Here, we have characterized an exceptionally large microvirus, Ebor, and provide crucial insights into long-standing mechanistic questions. Here, we report the structural analysis of the genome delivery process of a Microviridae phage, Ebor, along with its discovery and characterization. This phage, infecting a model aquatic Alphaproteobacterium Rhodobacter capsulatus, belongs to the microvirus taxon ‘Tainavirinae’ and recognizes the host via five Gokushovirinae-like trimeric protrusions. The capsid exhibits the triangulation number of T=1, being made of 60 copies of the major capsid protein. The core of the major capsid protein contains an 8-stranded antiparallel β-barrel (single jelly-roll fold), the fold shared among all Microviridae.

We isolated two Ebor variants exhibiting different stability during cryo-EM sample preparation. Nanopore sequencing showed a single nucleotide polymorphism leading to S120R amino acid replacement in the major capsid protein. Thus, we designated these variants S120 and R120. Variant R120 virions were purified using CsCl gradient, vitrified and imaged using cryo-EM, yielding stable native particles. Single particle reconstruction produced an icosahedrally averaged map of Ebor at 3.2 Å resolution. The capsid shell has an external diameter of 28 nm and an internal diameter of 25.1 nm. The internal diameter is 3.2 to 4.6 nm larger compared to other determined capsid structures of Microviridae members, allowing Ebor to accommodate larger genome. A striking characteristic of the capsid is the presence of elongated protrusions situated at its three-fold symmetry axes, reaching out 9 nm from its surface. These extensions are formed by loops composed of residues 184-254 from three neighbouring subunits of the major capsid protein. The model showed the tip of the protrusion possesses a positive electrostatic potential, contrary to the negative potential of the capsid’s penton exterior.

> MSYQTKRNVRREARTLMGRFKAGKLAPVMAVPVKGSEGGMLSQSVSFELDPIAGRMATPITAEMCAVFVPVQACDALKNPEADYAGMTEIVREKLLSGNPLFVLEPETDVSKRCGVNPRRNNGLMRVNEIVRLAHNCAVNFLRRRRYVDAVQLTAANHSTTPAILSQTVLDRFNGALDPDPNVNGAVQLSMPDMRLPVASDAEKAVTAPLTVKRGNENRRLDAGISRLAAAEVAAATDAALYAVFGGREAGNVSLTDFYNAQKMDELTRVMRKICDDNPEYGEEMVLRWAHGLSVDPGRVPFLLAEKSVVLGRQIIGATDTAGVEDGVKRSDMAAQLSFTVPIPTTELGGIIVTFACIKPDETLSSQPHPILADHWRLDNFVADELALDPQPVMARELDYKVAQANETTVVFYTGLNELKKTYVSYGLCRALDPNTVESKNAVWQLEVPLSVTPETVLYPADLPQYPFADQQAEVCTYVVQSTAVMPTPMIFGPSPVEQLAVIETEDLFED Here, we have described a global mapping of structure–function relationships among the members of the tautomerase superfamily (TSF)4 (3, 4). From a structural perspective, the functionally diverse members of the TSF share a small, structurally similar core domain that comprises a β-α-β motif. All biochemically characterized enzymes in the superfamily fall into five reaction types, each of which uses the N-terminal proline either as a general base or a general acid. The domain structure of the TSF is relatively simple, with nearly all of the members represented by either a single β-α-β structural motif or as fusion proteins composed of two of these subdomains.

The percent identity for each pair of sequences along the similarity path is 42% between 4-OT and the Fused 4-OT, 41% between Fused 4-OT and Linker 2, 26% between Linker 2 and Linker 1, 31% between Linker 1 and CgX, and 33% between CgX and cis-CaaD. Among the characterized fusion proteins of the TSF, only two enzymes showed substantial 4-OT activity, Fused 4-OT and Linker 2. Indeed, both Fused 4-OT and Linker 2 were shown to be proficient tautomerases with 2-HM, whereas Linker 1, cis-CaaD, and CgX showed no activity. Compared with 4-OT, Linker 2 exhibited only a 2-fold drop in kcat/Km, whereas Fused 4-OT showed a 23-fold drop in kcat/Km. Linker 2 shows a trace of cis-CaaD activity. There was a stepwise loss of this activity going from 4-OT and the 4-OT–like enzymes (Fused 4-OT and Linker 2) to Linker 1, CgX, and ultimately cis-CaaD. Especially interesting is that two of the key structural connections linking the 4-OT and cis-CaaD subgroups, Fused 4-OT and Linker 2, also exhibit multiple links to the MIF and MSAD subgroups as well as links between the cis-CaaD subgroup and the MIF and MSAD subgroups. We speculate that the central position of Fused 4-OT and Linker 2 in the structure similarity network offers a starting point for new studies aimed at addressing the evolution of the contemporary TSF subgroups from an ancient scaffold.

>PYVTISATEGLSAEKKKQLLERSSDAVVQSIGAPLASVRVMLHELPGGHYLNAGQFNTPGLMFVVDFIEGRTEEQRNALIAALSKTGTETTGIPESEVRVRLLDFPKANMGMAGGISAKAMGR[6x]1-[(2S,3aS,4S,6R,6aR)-2-hydroxy-6-(hydroxymethyl)-2-oxidotetrahydrofuro[3,4-d][1,3,2]dioxaphosphol-4-yl]pyrimidine-2,4(1H,3H)-dione 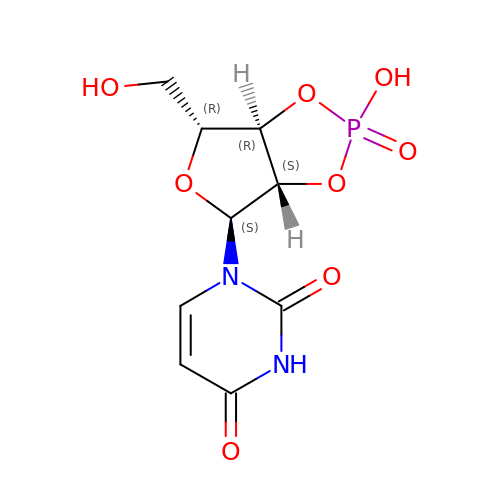| C9 H11 N2 O8 P | HWDMHJDYMFRXOX-GVYWOMJSSA-N6-(1H-pyrazolo[3,4-b]pyridin-5-yl)-4-pyridin-4-ylquinoline | C20 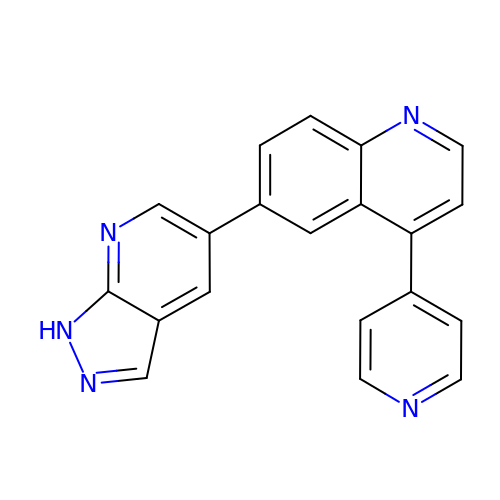H13 N5 | PYHJWHYHRSDRDJ-UHFFFAOYSA-N> WHRGTLSLLCSSCRYVVRKWHVPILGVDCNANPRHKQALSVPA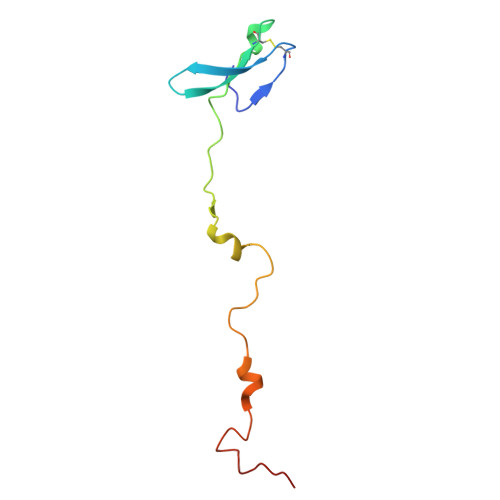PRSRGIPKHLYPFLVGKQYPRHPRWRQAFTHRSRMGKYKPQVARN>MGSSHHHHHHSSGLQGTENLYFQSHMTILVVTGTGTGVGKTVVCAALASAARQAGIDVAVCKPVQTGTARGD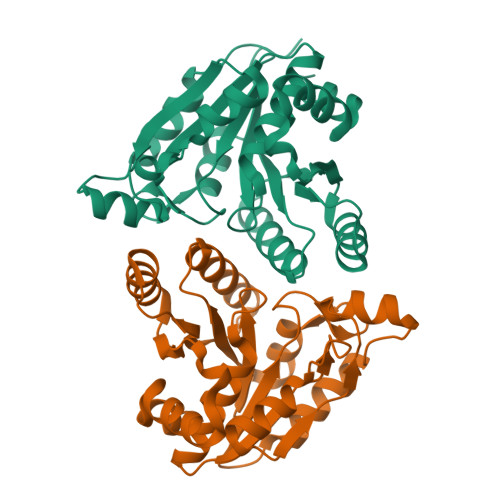DDLAEVGRLAGVTQLAGLARYPQPMAPAAAAEHAGMALPARDQIVRLIADLDRPGRLTLVEGAGGLLVELAEPGVTLRDVAVDVAAAALVVVTADLGTLNHTKLTLEALAAQQVSCAGLVIGSWPDPPGLVAASNRSALARIAMVRAALPAGAASLDAGDFAAMSAAAFDRNWVAGLVG[4x]> ENALLRYLL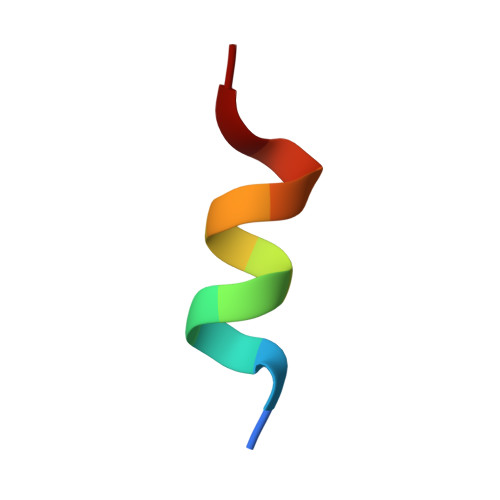DKD>MSVVSQVILQADDQLRYPTSGELKGIQAFLTTGAQRIRIAETLAENEKKIVDQAQKQLFKKHPEYRAPGGNAYGQRQYNQCLRDYGWYLRLVTYGVLAGNKEPIETTGLIGVKEMYNSLNVPVPGMVDAVTVLKDAALGLLSAEDANETAPYFDYIIQFMSHHHHHH[6x];>MQDAITAVINSADVQGKYLDGAAMDKLKSYFASGELRVRAASVISANAATIVKEAVAKSLLYSDVTRPGGNMYTTRRYAACIRDLDYYLRYATYAMLAGDASILDERVLNGLKETYNSLGVPIS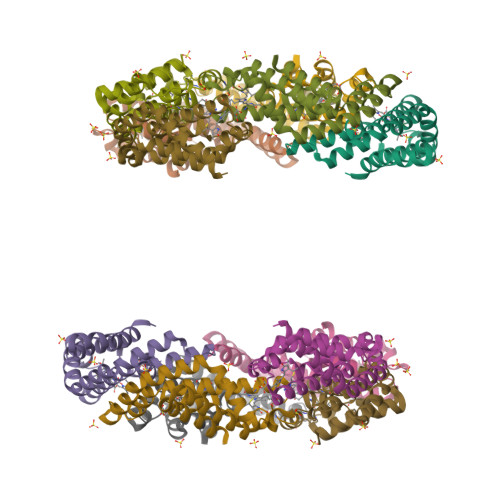STVQAIQAIKEVTASLVGADAGKEMGVYLDYICSGLS[6x]>[2x]MDHAEENEILAATQRYYVERPIFSHPVLQERLHTKDKVPDSIADKLKQAFTCTPKKIRNIIYMFLPITKWLPAYKFKEYVLGDLVSGISTGVLQLPQGLAFAMLAAVPPIFGLYSSFYPVIMYCFLGTSRHISIGPFAVISLMIGGVAVRLVPDDIVIPGGVNATNGTEARDALRVKVAMSVTLLSGIIQFCLGVCRFGFVAIYLTEPLVRGFTTAAAVHVFTSMLKYLFGVKTKRYSGIFSVVYSTVAVLQNVKNLNVCSLGVGLMVFGLLLGGKEFNERFKEKLPAPIPLEFFAVVMGTGISAGFNLKESYNVDVVGTLPLGLLPPANPDTSLFHLVYVDAIAIAIVGFSVTISMAKTLANKHGYQVDGNQELIALGLCNSIGSLFQTFSISCSLSRSLVQEGTGGKTQLAGCLASLMILLVILATGFLFESLPQAVLSAIVIVNLKGMFMQFSDLPFFWRTSKIEL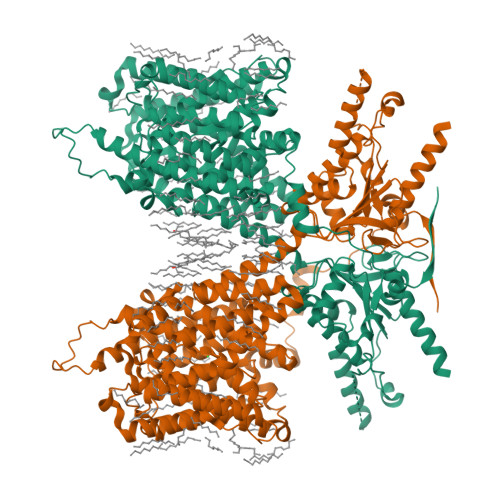TIWLTTFVSSLFLGLDYGLITAVIIALLTVIYRTQSPSYKVLGKLPETDVYIDIDAYEEVKEIPGIKIFQINAPIYYANSDLYSNALKRKTGVNPAVIMGARRKAMRKYAKEVGNANMANATVVKADAEVDGEDATKPEEEDGEVKYPPIVIKSTFPEEMQRFMPPGDNVHTVILDFTQVNFIDSVGVKTLAGIVKEYGDVGIYVYLAGCSAQVVNDLTRNRFFENPALWELLFHSIHDAVLGSQLREALAEQEASAPPSQEDLEPNATPATPEALEVLFQ2-[[(2~{R})-2-azanyl-3-[(3~{S})-3-methyl-1-oxidanyl-hexan-3-yl]sulfanyl-propanoyl]amino]ethanoic 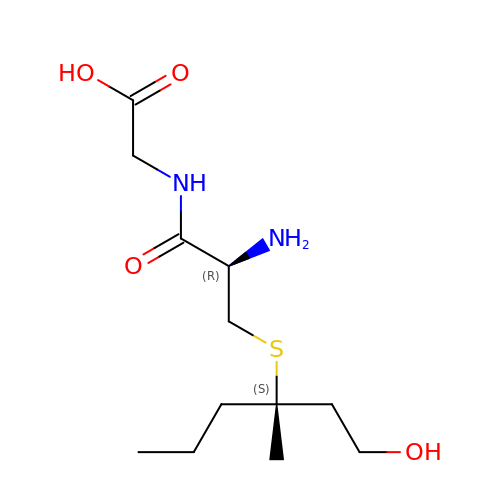acid | C12 H24 N2 O4 S | FIKNGFBNGIHRJV-CABZTGNLSA-N>[2x]MPKTLTEKLNAIKAAGKGIFVPYIMAGDHEKGLDGLAETIHFLEDLGVSAIEVGIPFSDPVADGPVIEEAGLRSLAHGTSTQALVETLKTIETEIPLVIMTYFNPLFQYGVENFVKDLADTAVKGLIIPDLPHEHANFVEPFLANTDIALIPLVSLTTGIERQKELIEGAEGFIYAVAINGVTGKSGNYRADLDKHLAQLHQVADIPVLTGFGVSSQADLERFNAVSDGVIVGSKIVKALHQGEPIQDFIRQAVAYQK;>SNAQEPNKDGFYGKF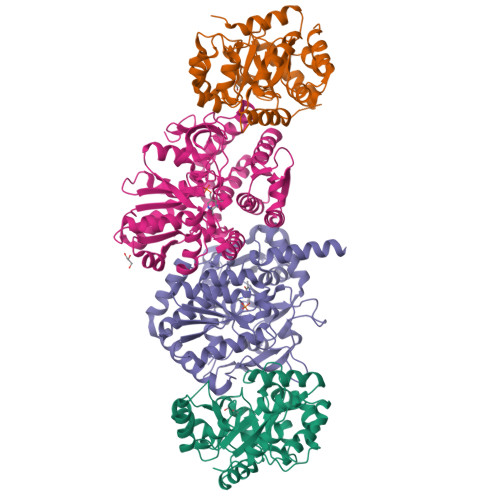GGRFVPETLMTAVLELEKAYRESQADPSFQEELNQLLRQYVGRETPLYYAKNLTQHIGGAKIYLKREDLNHTGAHKINNALGQVWLAKRMGKKKIIAETGAGQHGVATATAAALFNMECTIYMGEEDVKRQALNVFRMELLGAKVEAVTDGSRVLKDAVNAALRSWVANIDDTHYILGSALGPHPFPEIVRDFQSVIGREAKQQYRDLTGRDLPDALVACVGGGSNAIGLFHPFVEDESVAMYGTEAAGLGVDTEHHAATLTKGRPGVLHGSLMDVLQDAHGQILEAFSISAGLDYPGIGPEHSHYHDIKRASYVPVTDEEALEGFQLLSRVEGIIPALESSHAIAFAVKLAKELGPEKSMIVCLSGRGDKDVVQVKDRLEADAAKKGEAHA[2x]>[2x]GANAMGVLISAVGDTDPFRNFHDGALIHIARKYRPEKVILIFSEHTAKKQGNIEKALFSIAPNYEPELIIHDPIISDNEVHIFDVMFQRFSDILQEYYTKEDEFILNLSSATPQIKSALFVINRLNGINVKAVQVSSPEHASNENIGHDNDENIDELIEVNKDNKVNFIDRTIEDNAEKFSQALLKKTARDFIEKFDYKAALDILDQLSDFPNLKSVREEIRDVVNCLSKQDVPKGLRHKKLKEEEQKILSAYLTIELQRERGNVSESFIRIKNLTEFILEDYIKKRYPGLIDEYCEDIQKYYLSLFDYSKLLKATKEFKLKRTIAPIIDMNSSRNKVAHSLSPLDSDAVKQLGIAMKTLKTLVREQYHFSQSDFNFYQDLNKILLTKLN

Csm6 ribonucleases bind cOA using a CARF (CRISPR-associated Rossmann Fold) domain, resulting in activation of a fused HEPN (Higher Eukaryotes and Prokaryotes Nucleotide binding) ribonuclease domain. Here we characterised the cyclic hexa-adenylate (cA6) activated Csm6’ ribonuclease from the industrially important bacterium Streptococcus thermophilus. StCsm6’ is symmetrical dimer, with each monomer displaying a CARF domain (residues 1–173), a central 6H domain (residues 174–239), and a HEPN domain (residues 240–386). In the dimer, each domain interacts with the equivalent domain in the other monomer, but they cross over each other at the 6H domains to give an ‘X’ arrangement.

Apo StCsm6’ proved to be extremely difficult to crystallize, and only a single crystal in a dehydrated drop of mother liquor following ∼1 year of incubation was obtained. Nevertheless, data on this crystal were collected to 3.54 Å resolution, and the structure solved by molecular replacement with the separate HEPN and CARF domains of the StCsm6’ complex structure used as the search models. Aside from a couple of disordered regions, the peptide backbone of apo StCsm6’ could be built with confidence, but far fewer side chains were modelled due to the low resolution of the data. The structure revealed that apo StCsm6’, like in the complex with cA6, is a symmetrical dimer in an ‘X’ arrangement. Strikingly, however, the overall structure for apo StCsm6’ and in complex with cA6 were markedly different, with an RMSD of 7.7 Å over 327 Cα atoms for the monomer and 4.9 Å over 441 Cα atoms for the dimer (however, there are 386 residues in the monomer and 772 residues in the dimer, meaning the RMSDs over the full length dimeric protein would be much higher). The monomeric form of the individual CARF, 6H and HEPN domains of StCsm6’ are very similar in the apo structure and in complex with cA6, with RMSD values of 1.4 Å or lower over the entirety of each domain. The only difference to note is that one of the loops in the CARF domain (residues 133–149), which encloses the active site in the complex with cA6, could not be modelled in the apo structure, presumably due to conformational flexibility in this region which may not be stabilized until cA6 is bound. Unfortunately, a number of the active site residues could not be modelled in the apo StCsm6’ structure; this could reflect the flexibility in this region prior to cA6 binding which forms the functional active site, but also could be a consequence of the lower resolution data. In the apo StCsm6’ structure, D80 sits in a solvent exposed position in the CARF domain, but upon binding of cA6 the rotation of the CARF domain brings D80 into close contact with the residues at the top of the 6H domain (residues 172–175). One caveat is that the EiCsm6 structure may have been influenced by the presence of a non-hydrolysable cA6 mimic bound to the CARF domains.>MTDTPFIRPDMKAFLEAIAAMAGPTLAEMTLEEARASYVALHGMADRPARELAVIRNLSCPGPAGDIPLRLYDARESREAGPVITFYHGGGFVIGDLDTHHNLCTEIAALMDLPVVAVDYRLAPEHPFPAAIEDCEAATRWVASSPSELGRTASGVIPIGDSAGGNATIVVSQLLGAKPADVPVVLQVPIFPLASDAVGSASLEAFAEGFVL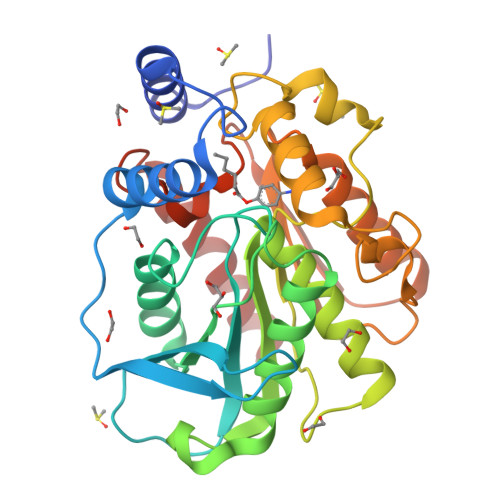TKASIEFFDTAYKADRADPRGFPILGDHTAAPPTIVATASLDPIRDSGRDYAKALVEAGRDVVYLEMEGVTHGFTNIRAAVPSTQGDLERIIAAMKMMLGTA[4x]>ATQGVFTLPANTRFGVTAFANSSATQTVKVLVNNETAATFTGQSTNNAVIGSQVLNSGGGGKVQIQVSVNGRSSDLVSAQVILANELNVALVGSEDSTDNDYNDAVVVINWPLG[4x]

Two soluble lectins, LecA and LecB, involved in adherence and biofilm formation have been described in P. aeruginosa. These lectins act as virulence factors through their carbohydrate binding ability. LecA and LecB bind to galactose and fucose, respectively, and their glycan-binding spectra cover a wide range of antigens (ABH, Lewis, P and I systems) present on human tissues or bacterial cell walls. The crystal structure of LecBPA7 was resolved to investigate the incidence of some amino acids changes on the structural organization of the LecB tetramers and sugar binding site.

One crystal of LecBPA7 complexed with Lewisa tetrasaccharide diffracted to 1.75 Å resolution and the structure could be solved in the P21 space group, with one tetramer per asymmetric unit. All of 114 amino acids could be located in the electron density, as well as the 8 calcium ions (2 per sites). The whole tetrasaccharide was clearly visible in three sites, and only one reducing glucose was disordered in monomer D. The structure of the LecBPA7/Lewisa complex was compared to the one previously obtained for LecBPAO1/Lewisa complex. Both structures share the same overall organization with rmsd (root-mean-square deviation) of 0.4 Å over the 456 amino acids of the tetramer. When looking at the binding site, the fucose residue adopts the same orientation in both lectins. No amino acids change involved in calcium coordination or in the hydrogen bonding to fucose was recorded. The other two sugar residues of Lewisa, i.e., galactose and GlcNAc, present a slight shift in response to the amino acids changes and the modified network of bridging water molecules. In LecBPA7, Ser97 (that replaces Gly97 in LecBPAO1) establishes a hydrogen bond with one of the two structural water molecules that bridges between the glycan ligand and the protein surface. The other variation, i.e., Ala24Gly results in an additional hydrophobic contact with the methyl group of Ala24 close to the CH2 group at C6 of the GlcNAc residue.> GSMSGIALSRLAQERKAWRKDHPFGFVAVPTKNPDGTMNLMNWECAIPGKKGTPWEGGLFKLRMLFKDDYPSSPPKCKFEPPLFHPNVYPSGTVCLSILEEDKDWRPAITIKQILLGIQELLNEPNIQDPAQAEAYTIYCQNRVEYEKRVRAQAKKF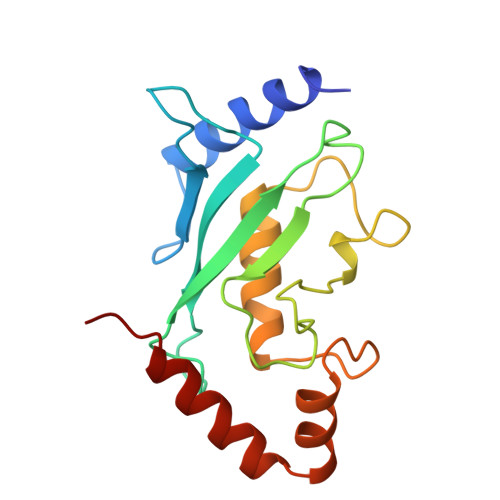APS> MSARHSRLIILGSGPAGYSAAVYAARANLKPTLIAGLQLGGQLTTTTEVDNWPGDPEGLTGPALMDRMQAHAE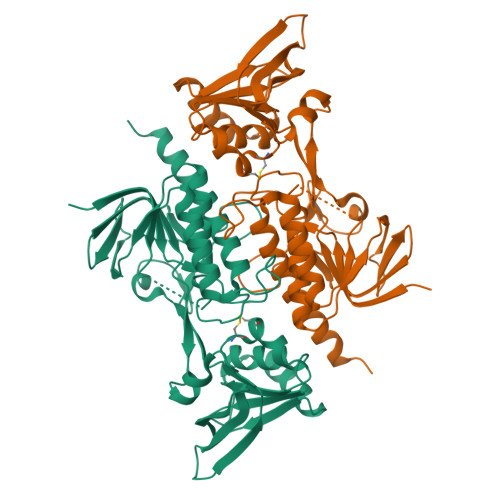RFGTELVYDHINEVDLNVRPFVLKGDMDEYTCDALIIATGATAQYLGLESEQKFMGQGVSACATCDGFFYKNQNVMVVGGGNTAVEEALYLSNIAEHVTLVHRRDSLRSEKILQDHLFAKEKEGKISIVWNHEVEEVLGDNTGVTGVRLKSTKDDSKQEVQVQGLFIAIGHKPNTSIFEGQLNLRDGYIQVQSGTSGNATATSVAGVFAAGDVADSIYRQAITSAGSGCMAALDAEKYLDNLLEHHHHHH> GSHMASMLNGKEFRFIGSNNYYMHYKSNRMIDSVLESARDMGIKVLRIWGFLDGESYCRDKNTYMHPEPGVFGVPEGISNAQNGFERLDYTIAKAKELGIKLIIVLVNNWDDFGGMNQYVRWFGGTHHDDFYRDERIKEEYKKYVSFLINHVNVYTGVPYREEPTIMAWELANELRCETDKSGNTLVEWVKEMSSYIKSLDPNHLVAVGDEGFFSNYEGFKPYGGEAEWAYNGWSGVDWKKLLSIETVDFGTFHLYPSHWGVSPENYAQWGAKWIEDHIKIAKEIGKPVV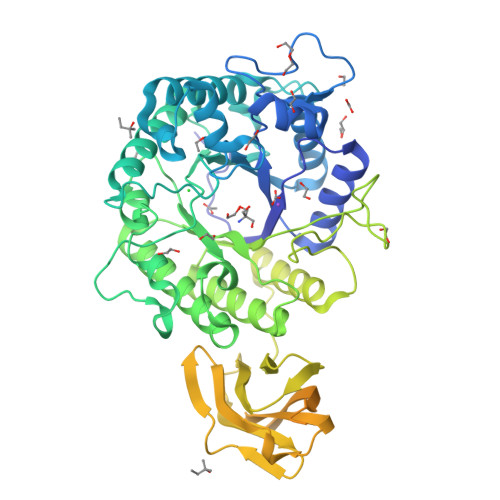LEEYGIPKSAPVNRTAIYRLWNDLVYDLGGDGAMFWMLAGIGEGSDRDERGYYPDYDGFRIVNDDSPEAELIREYAKLFNTGEDIREDTCSFILPKDGMEIKKTVEVRAGVFDYSNTFEKLSVKVEDLVFENEIEHLGYGIYGFDLDTTRIPDGEHEMFLEGHFQGKTVKDSIKAKVVNEARYVLAGKVDFSSPEEVKNWWNSGTWQAEFESPDIEWNSEVGNGALQLNVKLPGKSDWEEVRAARKFEKLSECEILEYDIYIPDVEGLKGRLRPYAVLNPGWVKIGLDMNNTSVESAEIVTFGGKEYRKFHVRIEFDKTAGVNELHIGIVGDHLKYNGPIFIDNVKLYTKEAE Here we report the single-particle cryo-electron microscopy structure of the native transmembrane channel-like protein 1 (TMC-1) mechanosensory transduction complex isolated from Caenorhabditis elegans. The two-fold symmetric complex is composed of two copies each of the pore-forming TMC-1 subunit, the calcium-binding protein CALM-1 and the transmembrane inner ear protein TMIE. CALM-1 makes extensive contacts with the cytoplasmic face of the TMC-1 subunits, whereas the single-pass TMIE subunits reside on the periphery of the complex, poised like the handles of an accordion. Single-particle reconstructions and molecular dynamics simulations show how the mechanosensory transduction complex deforms the membrane bilayer and suggest crucial roles for lipid–protein interactions in the mechanism by which mechanical force is transduced to ion channel gating.

Two of these classes represent the TMC-1 complex in different conformational states, designated the ‘expanded’ (E) and ‘contracted’ (C) conformations, both of which exhibit an overall resolution of 3.1 Å. Because the E conformation has a few more distinct density features than the C conformation, we focus on the E conformation in our initial discussion of the overall structure. The TMC-1 subunits in the E and C conformations have a similar overall structure, both including closed ion channels. In the C conformation, however, the TM10 helix is bent approximately 9° compared with that in the E conformation, and there is one additional helical turn of TM10 in the E conformation. Upon successively superimposing the TMC-1 subunits from the C and E complexes, we observed that in the E state, each half of the TMC-1 complex, composed of TMC-1, CALM-1 and TMIE subunits, is rotated by around 8° compared with the C state, by way of an axis of rotation that is located near the TMC-1 H7 and H8 helices and oriented approximately parallel to the membrane. Indeed, in comparing the C and E states, the amphipathic TMC-1 H3 helices move farther apart by approximately 11 Å, thus underscoring the magnitude of the conformational change. Of note, the E and C conformations generate distinct membrane deformation patterns. In particular, the E conformation induces a more pronounced membrane distortion (thickening and thinning) close to the protein, resulting in a longer-range membrane deformation propagation (around 50 Å away from the protein). The putative ion-conduction pathway appears to be closed, with a narrow pore blocked by three constrictions. Examination of the equilibrated membrane structure around the TMC-1 complex indicates a deep penetration and anchoring of the amphipathic, paddle H3 helix into the cytosolic leaflet of the bilayer.

>[2x]MQEAARRASLRKEHTPTNEKFGDLSKQDSLGERASSKLTLDDELYDILYAFGETDAFINKGDKQRETDEDGNPLTRQALLERIRQKKEVIGKLRCQAWSMTRKRRTLKLAQKYLEQHESKVSRSHLYMEEMRKRARLMKRSFSNFKTYLIPWESKIKRIESHFGSVVSSYFTFLRWIVFVNIMITLIALVFVVLPETLADSVANEGRFNRTKTRKQIPANERVHADELAVVWHYDGYLRYSPLFYGYYSDDPFLGNKIKYALPLAYFMVTLTIFAYSFFAILRKMAANARMSKLSGSKAEQYIFNWKLFTGWDYTIGNSETASNTVMAVVIKLRESIADIKKDAHGKFRLLQFSLRVFANIIICAMLGFSIYCIIFAVQKSQVQDDGNLFTKNQVPSVVSTITHVFPMIFDLIGKMENYHPRTALRAHLGRVLILYTVNYITLIFALFEKMTALRDRVNSTSTSSSHRTKRQQGGWNPNMQRPPPYASRAEVRQMSDFLAANTRRFQTVSQRTTRSVTTPFTVAPQFGPFNVNNPNAVFHNGTHSTSFESQILGPKALPIFTPPPRKYPGFTPGNVGQQFGGPDFPRNQVYTKSTPLPRVRTKPPWVYTTTHPPLVQNRAMTTTMSKSAKKGNSKNLDDDILLSNETIQMSEAALRRNHDGHNNDICWETIIGQEIVKLVTMDLIFTILSILVIDLFRGLWIKYCSSWWCWDIETTFPEYGEFKVAENVLHIINNQGMIWLGLFFAPLLPAINNIKLIILMYIRGWAVMTCNVPAREIFRASRSSNFYLGILLIWLLLCTLPVGFVIASMSPSRSCGPFARYQHFYTVVTREIEKRVDQTVLSYIRHIASPGVVIPIILFLILIIYFLFSLVRGLREANTDLQAQLVHERTEEKKKIFELAGGKKNKFEKDRDKKRSNDYIPLIEQRRREPWRQYHEMEADHALASDSSEESDINEDEDDERQPLTAYPLRAIETPPETLQVTAFHPSLGSLIENREMEDEESASGDQLPMIHKSVSFQGPSHMQMRQSISTESCSQISRSAIQVATPEEIRALLRPYLEAKYGIPYQHGIKSFPIDVHTPPNNTPSRRSSKYNSFVSLYEHTRDDHKNFVASTIKETDEDPGKSDKKQTSSKDVAPDFMPWPSADEARALREKMKSKTPLMLTKTTVEEKPKGGKSSESEFRPPVPIHRKYNIQTTEEENEEEETDSAPESSKKRFRISVSPTKTIAPASASRAQHKIVSQASSSSSIPHGRQPDPNKKASLVLPPLRAPRVQFDEDDSPRQID;>[2x]MGNNASSLSELNLFSKGGVFTREQLDEYQDCTFFTRKDIIRLYKRFYALNPHKVPTNMQGNRPAITTLTFEEVEKMPELKENPFKRRICEVFSEDGRGNLSFDDFLDMFSVFSEMAPLQLKLKYAFRIYDYDGDELLGHDDLSKMIRSLTRDELSDVEVEFIIERIIEEADLDGDSSINFAEFEHVVSRSPDFIRTFHIRI;>MPSGNEEINHLSALDQFVAPGLRLWMLIALVGGVLLIMIVIVCCFMRIRIPRTKRQIDLIAAKRKLRKSTKNSAEANAHNDERAQAIVMNSMPSGGGGGAPSTSSSRHTGSRIQSQV[2x]>GPMVEQMQQREQWCSEH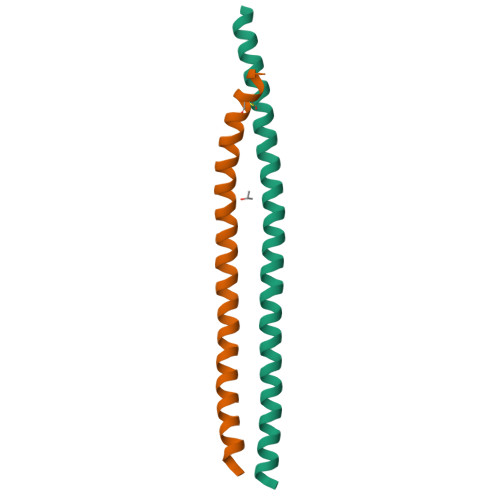LDTQKELLEEMYEEKLNILKESLTSFYQEEIQERDEKIEELEALLQEARQQSVAHQQS[2x]Leukotriene (LT) C4 synthase (LTC4S) catalyzes the conjugation of the fatty acid LTA4 with the tripeptide GSH to produce LTC4, the parent compound of the cysteinyl leukotrienes, important mediators of asthma. LTC4S is a trimeric integral membrane protein and a member of the MAPEG (membrane-associated proteins in eicosanoid and glutathione metabolism) family, which also includes three microsomal GSH S-transferases, 5-lipoxygenase activating protein, and microsomal prostaglandin E synthase 1 (9, 10). The crystal structure of human LTC4S has been solved and identified a unique horseshoe-shaped conformation of GSH bound at the active site by residues from two neighboring monomers. It was postulated that the lipid substrate LTA4 binds in a hydrophobic crevice between two monomers and that Trp-116 could act as a “molecular ruler” for binding of LTA4 with its ω-end buried under the aromatic side chain.

We exchanged Trp-116 in LTC4S for an Ala or Phe residue and analyzed the effects on catalysis and kinetic parameters. Considering the inherent variability that comes with enzyme assays with highly unstable lipid substrates, no major kinetic alterations were observed, thus demonstrating that Trp-116 is not essential for catalysis. To further probe the role of Trp-116 for the positioning of LTA4 at the active site, we solved the structures of W116A and W116F LTC4S in complex with analog I, at 2.7 and 2.4 Å resolution, respectively. Comparing the omit map densities between the WT structure and the W116A mutant, it is clear that the acyl chain of analog I is less ordered (data not shown), which coincides well with previous proposals that the function of Trp-116 is to anchor the tail of LTA4. Hence, Trp-116 appears to aid in the positioning of the ω-end of LTA4 but this substrate-enzyme interaction seems to have very little, if any, impact on substrate turnover. The sulfur in analog I in the W116A and W116F mutants shows a larger shift of ∼7.1 Å. In the W116A and W116F mutants, the three terminal carbons shift by ∼3.5 Å upwards toward the position of the Trp-116. This is most likely due to the larger space available in the absence of the tryptophan residue. The increased Km values of W116A/W116F for GSH are probably indirect effects of changes in LTA4 binding.

> MHHHHHHKDEVALLAAVTLLGVLLQAYFSLQVISARRAFRVSPPLTTGPPEFERVYRAQVNCSEYFPLFLATLWVAGIFFHEGAAALCGLVYLFARLRYFQGYARSAQLRLAPLYASARALALLVALAALGLLAHFLPAALRAALLGRLRTLLPWA>MGDNIVLYYFDARGKAE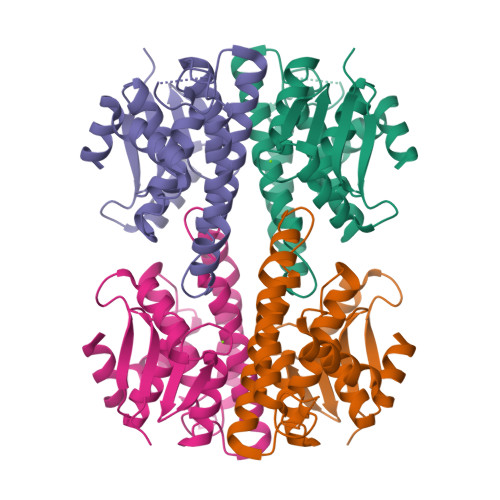LIRLIFAYLGIEYTDKRFGVNGDAFVEFKNFKKEKDTPFEQVPILQIGDLILAQSQAIVRYLSKKYNICGESELNEFYADMIFCGVQDIHYKFNNTNLFKANETTFLNEDLPKWSGYFEKLLKKNHTNNNNDKYYFVGNNLTYADLAVFNLYDDIETKYPSSLKNFPLLKAHNEFISNLPNIKNYITNRKESVY[2x]> GPLGSMSGTLVQRLKLILSGGNLRCSDGE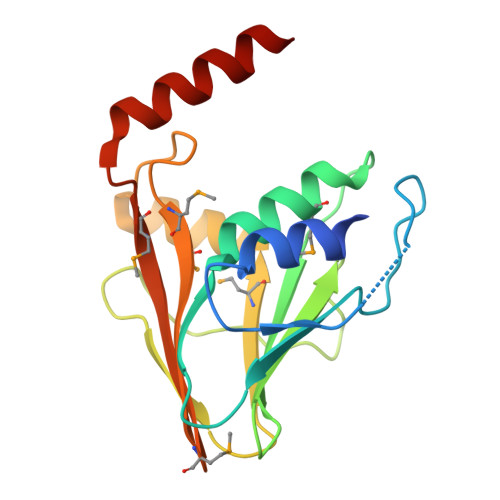TACDPERPPTRCVFQVHGQDGSNDTFPLEYVLRLMRSWAHVPCDPYVRVQNTGVSVLFQGFFFRPADAPLAAITAEHNNVILASTHSTGMSLSALDDIKRAGGVDTRPLRAMMSVSCFVRMPRVQLSFRFMGPDDASQTQRLLDRAELRQRS>MAESMVPAPPQLAAKSYVLMDGESGQVLVENNGDQRLPPASLTKLMTAYIATKEIEAGRIGENDLVTVSEHAWRTGGSRMFIKVGSQVSVSDLLHGIIIQSGNDASVALAEHIAGSEDAFADMMNTTAQKLGLTNSHFMDATGLPNPDHYSSARDMAVLARAIIYGEPSHYAIYAQKEFLW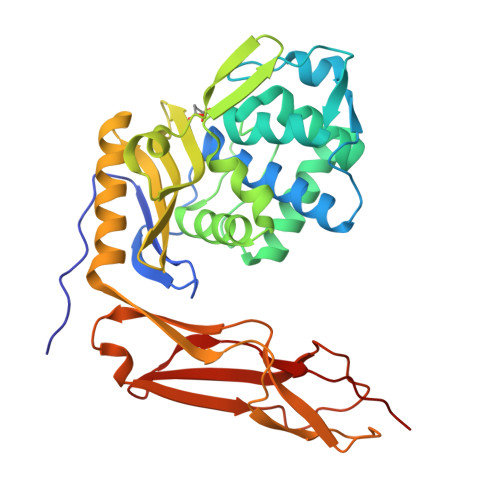NNIKQPNRNLLLWRDKTVDGLKTGHTDEAGYCLVASAVRDGQRMIAVVFGTNSEQARAAETQKLLTYGFRFFESRNFYKKGTELTKGLVWKGSEHEVKAGLAEDLTMTLPRGQMQKLQASMVLEPQLMAPIQQGQVIGKVEVKLDDKVIRSADLVALNAVEEGGF[2x]> MDAKKVAKKAAIQAARRITELAQVLVELLKEALKLDLTQEMRKKLIERYAAAIIRAIGDINNAIYQAKQEAEKLKKAGLVDSDQL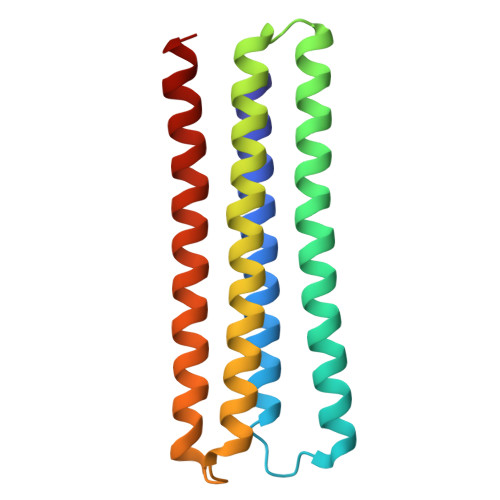DALLRALDELQKVASKAANQLGRLFEEALKRLDKDNGGEEEKDRTAKWFEFEARAIEIALRLAAIGDVFDLEKEWRKLK>[2x]GGSMASMDFPQHSQHVLEQLNQQRQLGLLCDCTFVVDGVHFKAHKAVLAACSEYFKMLFVDQKDVVH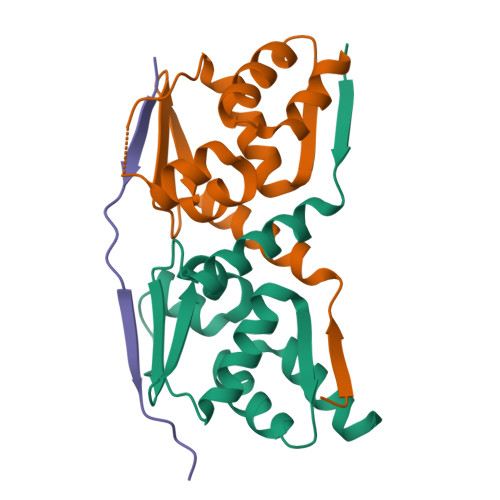LDISNAAGLGQVLEFMYTAKLSLSPENVDDVLAVATFLQMQDIITACHALKSLA;> SHDQHAVLVLQPAVEAFFLVHATERESK>[2x]AMKNFRLSEKEVKTLAKRIPTPFLVASLDKVEENYQFMRRHLPRAGVFYAMKANPTPEILSLLAGLGSHFDVASAGEMEILHELGVDGSQMIYANPVKDARGLKAAADYNVRRFTFDDPSEIDKMAKAVPGADVLVRIAVRNNKALVDLNTKFGAPVEEALDLLKAAQDAGLHAMGICFHVGSQSLSTAAYEEALLVARRLFDEAEEMGMHLTDLDIGGGFPVPDCKGLNVDLAAMMEAINKQIDRLFPDTAVWTEPGRYMCGTAVNLVTSVIGTKTRGEQPWYILDEGIYGCFSGIMYDHWCYPLHCFGKGNKKPSTFGGPSCDGIDVLYRDFMAPELKIGDKVLVTEMGSYTSVSATRFNGFYLAPTIIFEDQPEYAARLTEDDDVKKKAAV

Lysine decarboxylase (LDC) is an important enzyme for maintenance of pH homeostasis and the biosynthesis of cadaverine. In addition, LDC plays a crucial role in the synthesis of cadaverine, an important industrial platform chemical. We also reported that, due to the flexible PLP binding site, the protein undergoes an open/closed conformational change at the PLP binding site depending on the PLP binding. Especially, two loops located in the vicinity of the PLP binding site, the PLP stabilization loop (PS-loop) and the regulatory loop (R-loop), undergoes a significant structural movement depending on the PLP binding.

We selected two target residues, Ala225 and Thr302 located at the R-loop and its neighboring region, respectively, and generated the SrLDCA225C/T302C mutant by replacing these residues to cysteine. These two residues contribute to the stabilization of the R-loop in the closed conformation by forming a hydrogen bond and are considered to be located in a suitable distance to form a disulfide bond each other when mutated to cysteine. To structurally confirm the enhanced stability of the PLP binding site in mutant SrLDCA225C/T302C is derived from the introduced disulfide bond, we determined its crystal structure at 1.8 Å resolution. As expected, a disulfide bond was observed between A225C and T302C, and the PS-loop and the R-loop of the mutant showed the closed conformation. Moreover, When we compared the B-factors of the PS-loop and the R-loop in SrLDCA225C/T302C with those in the wild-type SrLDC, B-factors for the PS-loop and the R-loop of the SrLDCA225C/T302C mutant were much lower than those of both the open and closed forms of SrLDCWT, indicating that the stability of the loop regions are significantly enhanced by the engineered disulfide bond. Interestingly, the active site loop (AS-loop), that are known to be highly disordered in both the open and closed forms of SrLDCWT, showed a clear electron density map in the SrLDCA225C/T302C mutant. The loop is stabilized by extensive hydrogen bonds with the PS-loop. In particular, the Val146 residue in the AS-loop is positioned in the vicinity of the substrate and seems to be involved in the stabilization of the hydrocarbon part of the lysine substrate. Interestingly, we observed the clear electron density for PLP cofactor even without addition of PLP in the crystallization solution, indicating that the SrLDCA225C/T302C mutant retained the PLP cofactor during purification and crystallization procedures. SrLDCWT and the SrLDCA225C/T302C mutant showed Kd values of 72 and 21 μM, respectively, indicating that the Kd value of the SrLDCA225C/T302C mutant was increased in 3.4 fold compared with that of SrLDCWT.>MASLSRFRGCLAGALLGDCVGSFYEAHDTVDLTSVLRHVQSLEPDPGTPGSERTEALYYTDDTAMARALVQSLLAKEAFDEVDMAHRFAQEYKKDPDRGYGAGVVTVFKKLLNPKCRDVFEPARAQFNGKGSY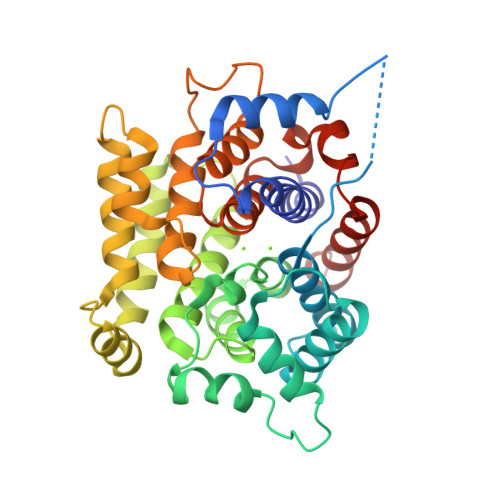GNGGAMRVAGISLAYSSVQDVQKFARLSAQLTHASSLGYNGAILQALAVHLALQGESSSEHFLKQLLGHMEDLEGDAQSVLDARELGMEERPYSSRLKKIGELLDQASVTREEVVSELGNGIAAFESVPTAIYCFLRCMEPDPEIPSAFNSLQRTLIYSISLGGDTDTIATMAGAIAGAYYGMDQVPESWQQSCEGYEETDILAQSLHRVFQKS[2x]>GSHMGPSLDFALSLLRRNVRQVQTDQGHFTMLGVRDRLAVLPRHSQPGKTIWIEHKLVNVLDAVELVDEQGVNLALTLITLDTNEKFRDITKFIPENISTASDATLVINTEHMPSMFVPVGDVVQYGFLNLSGKPTHRTMM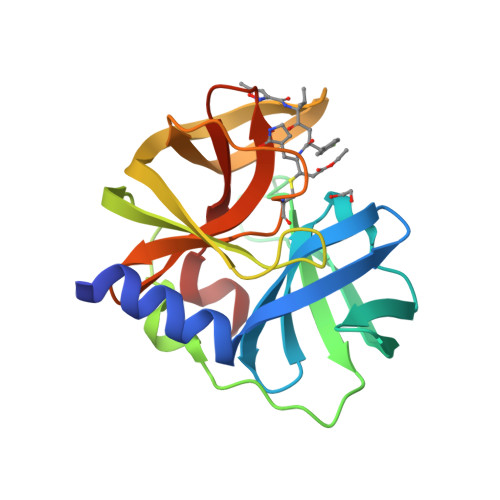YNFPTKAGQCGGVVTSVGKIIGIHIGGNGRQGFCAGLKRSYFASEQ[2x]>[2x]MDEESDLKDHRDKWNKYYGVSPDQLSKDLFDKVSPEQIKNSPYQSVGALFVKGEAVATGVFIGKNTVVTNHHIAKEAKNNPSKIIFSPGAHADESNTGTVLPHGTFEASEIIDAPFGTGVDISVIIFKPNAEGKSIGDVIKAADLGNSNSLKKGDTANLIGYPYDFDSKNMYRSQVE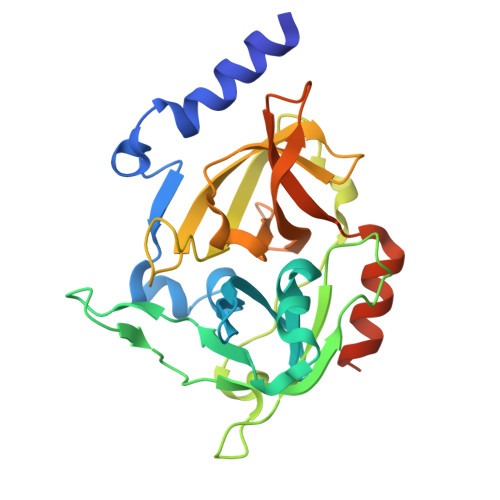FQSTDFGLKYYGYTVPGNSGSGIFNSEGKFVGLHIGKAKHINSQNEINYAVSFNDFLIRDLKQLIKGGENLYFQSHHHHHH6-chloranyl-3-[3-[(1~{S})-1-(4-chlorophenyl)ethyl]-5-phenyl-imidazol-4-yl]-~{N}-[2-[4-(2-oxidanylidene-1,3-oxazinan-3-yl)piperidin-1-yl]pyridin-3-yl]-1~{H}-indole-2-carboxamide | C40 H37 Cl2 N7 O3 | 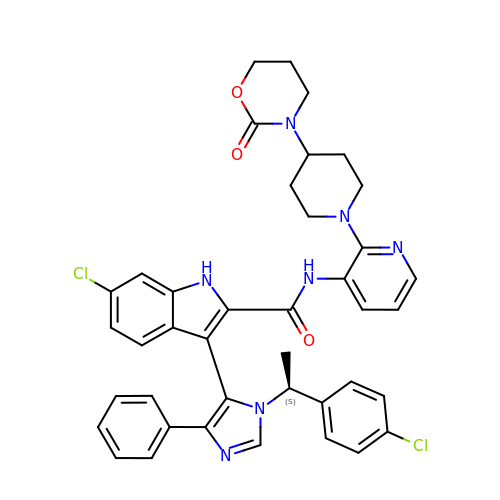PEGKHNWZGSKUJH-VWLOTQADSA-N> CPAYSAYL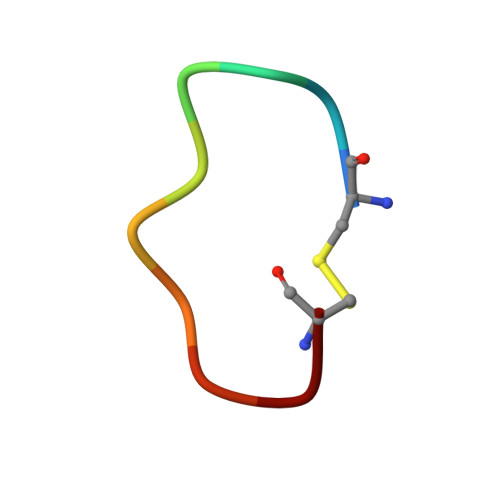DC> GC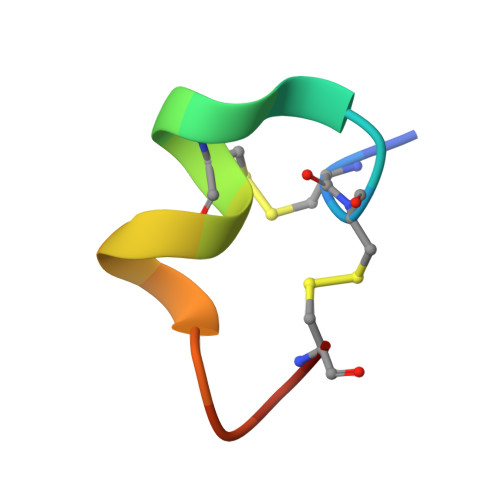CSLPPCALSNPDYCX>MKKGHHHHHHGSERTGTQPLGVQGLTEEQRMMIRELMDAQMKTFDTTFSHFKNFRLPGVLSSGCELPESLQAPSREEAAKWSQVRKDLCSLKVSLQLRGEDGSVWNYKPPADSGGKEIFSLLPHMADMSTYMFKGIISFAKVISYFRDLPIEDQISLLKGAAFELCQLRFNTVFNAETGTWECGRLSYCLEDTAGGFQQLLLEPMLKFHYMLKKLQLHEEEYVLMQAISLFSPDRPGVLQHRVVDQLQEQFAITLKSYIECNRPQPAHRFLFLKIMAMLTELRSINAQHTQRLLRIQ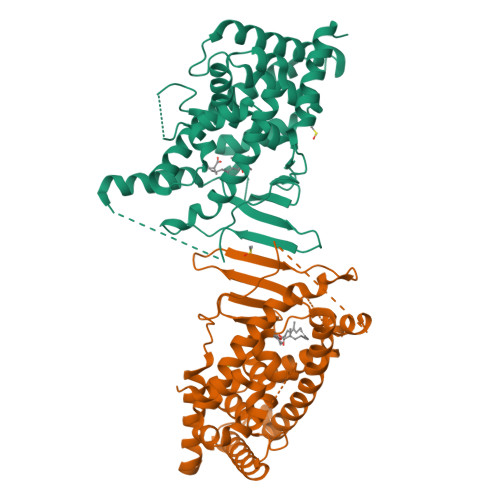DIHPFATPLMQELFGITGSGGSGGSSHSSLTERHKILHRLLQEGSPS[2x]>[4x]MLPKLVITHRVHEEILQLLAPHCELITNQTDSTLTREEILRRCRDAQAMMAFMPDRVDADFLQACPELRV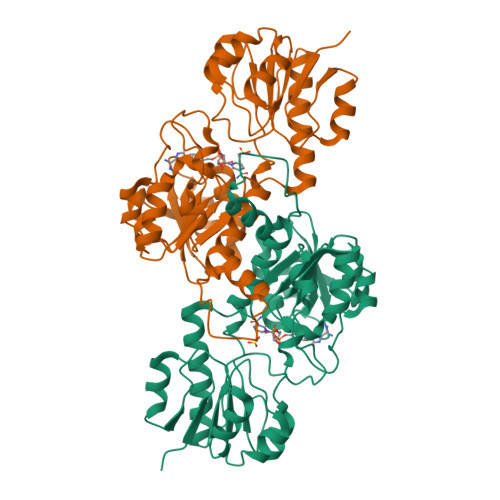IGCALKGFDNFDVDACTARGVWLTFVPDLLTVPTAELAIGLAVGLGRHLRAADAFVRSGKFRGWQPRFYGTGLDNATVGFLGMGAIGLAMADRLQGWGATLQYHEAKALDTQTEQRLGLRQVACSELFASSDFILLALPLNADTLHLVNAELLALVRPGALLVNPCRGSVVDEAAVLAALERGQLGGYAADVFEMEDWARADRPQQIDPALLAHPNTLFTPHIGSAVRAVRLEIERCAAQNILQALAGERPINAVNRLP> MRRITGITVIKDHQSEDRPALPYGVVELANFRDLHQQVRTIHYEDIEDSDNGEGFPEVQATPEVEQEWVFLVQVYGPGGLDYLRKVAAAFHVN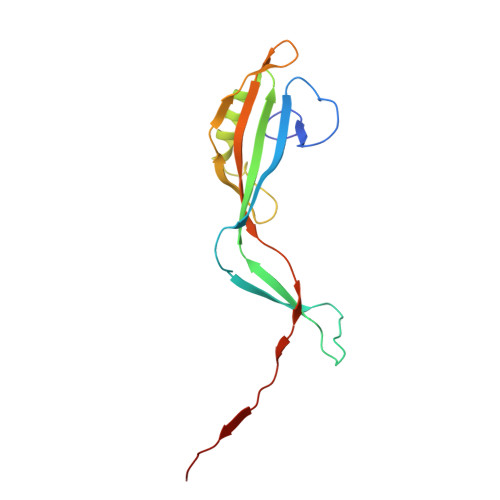QVNDLPGSLVIHEVAQINSIPEFLGERWEKRAQTNITLRGMSTDGFKVDVIEQHVINVTGERA>[2x]MNTIAWLGRLVIERIRGIGVAALMLLQIIFSLPSAGGFGRFVYQMHRVGVMSLLIITVSGLFIGLVLGLQGYSILVNVGSESMLGTMVSLTLLRELAPVVAALLFAGRAGSALTAEIGSMKQSEQLASMEMIGVDPLKQIVSPRLWAGIVSLPMLTVIFAAIGIVGGKLVGVDFLGVDEGSFWSGMQNNVQFGHDVVNGIIKSIVFALLCTWIAVFQGYACDPTPEGIATAMTRTVVYSSLCVLGFDFVLTAVMFG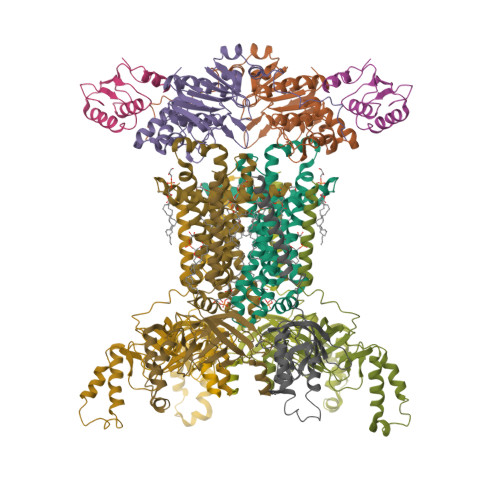GI;>[2x]MMNNKTPLSTQSLIEVKNLSFNRGERVIYDNISLNIRRGQITAIMGPSGTGKTTLLRLIGGQLVPDQGEVLLDGKDIAQMSRQELFAARARMGMLFQSGALFTDMSVYENVAFPIRAHTKLSENLIAELVALKLESVGLRGTEQLMPTELSGGMNRRVALARAIALDPDLIMYDEPFAGQDPIVKGVLTRLIRSLREALDLTTIIVSHDVPETLSIADYIYVVAEGKIQGEGTPEELQAYASPFVKQFLTGSAEGPVEYQFSHQAYLDNEVRP;>VVQYLNQELVVSGKIDFENAEQQYQAGLAIIKKQTSFPLIVDLKQLEHGNTLALAVLVQWLRQTPQKSGLHFKNVPEKMLKIIQACHLQEDLHLVLEHHHHHH[2x];>MKSRTSELAVGIFVIIFGIALFFLAMKVSGLVGTNLSDGYTMKAQFDNVNGLKPRAKVTMSGVTIGRVDSITLDPVTRLATVTFDLDGKLTSFNAEQLKEVQKNALDELRYSSDYTQATPAQQKTMEQQLISNMNSITSIDEDAYIMVATNGLLGEKYLKIVPGGGLNYLKRGDTISNTQGTMDLEDLISKFITGGGAGKVAAGSSSAEEKAPASTDSSAQPSFVE[6x]> KEGYLMDHEGCKLSCFIRPSGYCG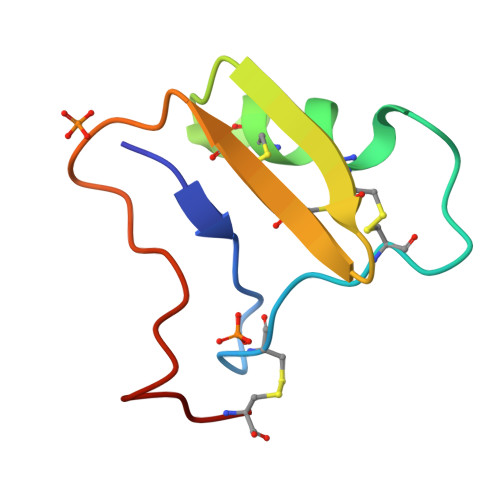RECGIKKGSSGYCAWPACYCYGLPNWVKVWDRATNKC> MAQILPIRFQEHLQLQNLGINPANIGFSTLTMESDKFICIREKVGEQAQVVIIDMNDPSNPIRRPISADSAIMNPASKVIALKAGKTLQIFNIEMKSKMKAHTMTDDVTFWKWISLNTVALVTDNAVYHWSMEGESQPVKMFDRHSSLAGCQIINYRTDAKQKWLLLTGISAQQNRVVGAMQLYSVDRKVSQPIEGHAASFAQFKMEGNAEESTLFCFAVRGQAGGKLHIIEVGTPPTGNQPFPKKAVDVFFPPEAQNDFPVAMQISEKHDVVFLITKYGYIHLYDLETGTCIYMNRISGETIFVTAPHEATAGIIGVNRKGQVLSVCVEEENIIPYITNVLQNPDLALRMAVRNNLAGAEELFARKFNALFAQGNYSEAAKVAANAPKGILRTPDTIRRFQSVPAQPGQTSPLLQYFGILLDQGQLNKYESLELCRPVLQQGRKQLLEKWLKEDKLECSEELGDLVKSVDPTLALSVYLRANVPNKVIQCFAETGQVQKIVLYAKKVGYTPDWIFLLRNVMRISPDQGQQFAQMLVQDEEPLADITQIVDVFMEYNLIQQCTAFLLDALKNNRPSEGPLQTRLLEMNLMHAPQVADAILGNQMFTHYDRAHIAQL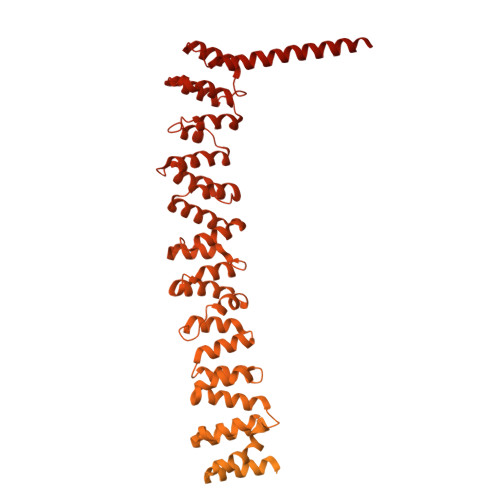CEKAGLLQRALEHFTDLYDIKRAVVHTHLLNPEWLVNYFGSLSVEDSLECLRAMLSANIRQNLQICVQVASKYHEQLSTQSLIELFESFKSFEGLFYFLGSIVNFSQDPDVHFKYIQAACKTGQIKEVERICRESNCYDPERVKNFLKEAKLTDQLPLIIVCDRFDFVHDLVLYLYRNNLQKYIEIYVQKVNPSRLPVVIGGLLDVDCSEDVIKNLILVVRGQFSTDELVAEVEKRNRLKLLLPWLEARIHEGCEEPATHNALAKIYIDSNNNPERFLRENPYYDSRVVGKYCEKRDPHLACVAYERGQCDLELINVCNENSLFKSLSRYLVRRKDPELWGSVLLESNPYRRPLIDQVVQTALSETQDPEEVSVTVKAFMTADLPNELIELLEKIVLDNSVFSEHRNLQNLLILTAIKADRTRVMEYINRLDNYDAPDIANIAISNELFEEAFAIFRKFDVNTSAVQVLIEHIGNLDRAYEFAERCNEPAVWSQLAKAQLQKGMVKEAIDSYIKADDPSSYMEVVQAANTSGNWEELVKYLQMARKKARESYVETELIFALAKTNRLAELEEFINGPNNAHIQQVGDRCYDEKMYDAAKLLYNNVSNFGRLASTLVHLGEYQAAVDGARKANSTRTWKEVCFACVDGKEFRLAQMCGLHIVVHADELEELINYYQDRGYFEELITMLEAALGLERAHMGMFTELAILYSKFKPQKMREHLELFWSRVNIPKVLRAAEQAHLWAELVFLYDKYEEYDNAIITMMNHPTDAWKEGQFKDIITKVANVELYYRAIQFYLEFKPLLLNDLLMVLSPRLDHTRAVNYFSKVKQLPLVKPYLRSVQNHNNKSVNESLNNLFITEEDYQALRTSIDAYDNFDNISLAQRLEKHELIEFRRIAAYLFKGNNRWKQSVELCKKDSLYKDAMQYASESKDTELAEELLQWFLQEEKRECFGACLFTCYDLLRPDVVLETAWRHNIMDFAMPYFIQVMKEYLTKVDKLDASESLRKEEEQATETQPIVYGQPQLMLTAGPSVAVPPQAPFGYGYTAPPYGQPQPGFGYSM>[4x]MAEQTVEAPSVDARAWILM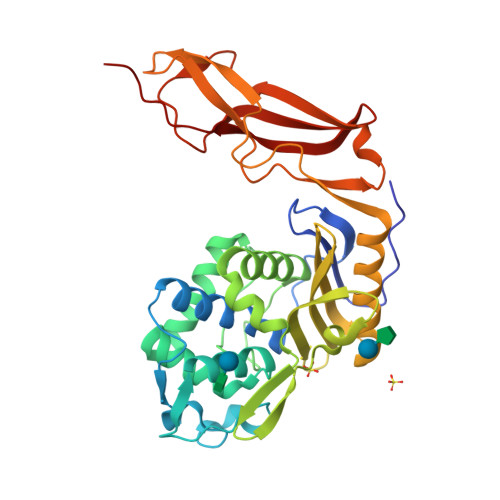DYASGKVLAEGNADEKLDPASLTKIMTSYVVGQALKADKIKLTDMVTVGKDAWATGNPALRGSSVMFLKPGDQVSVADLNKGVIIQSGNDACIALADYVAGSQESFIGLMNGYAKKLGLTNTTFQTVHGLDAPGQFSTARDMALLGKALIHDVPEEYAIHKEKEFTFNKIRQPNRNRLLWSSNLNVDGMKTGTTAGAGYNLVASATQGDMRLISVVLGAKTDRIRFNESEKLLTWGFRFFETVTPIKPDATFVTQRVWFGDKSEVNLGAGEAGSVTIPRGQLKNLKASYTLTEPQLTAPLKKGQVVGTIDFQLNGKSIEQRPLIVMENVEEGG>MNRQELITEALKARDMAYAPYSKFQVGAALLTKDGKVYRGCNIENAAYSMCNCAERTALFKAVSEGDTEFQMLAVA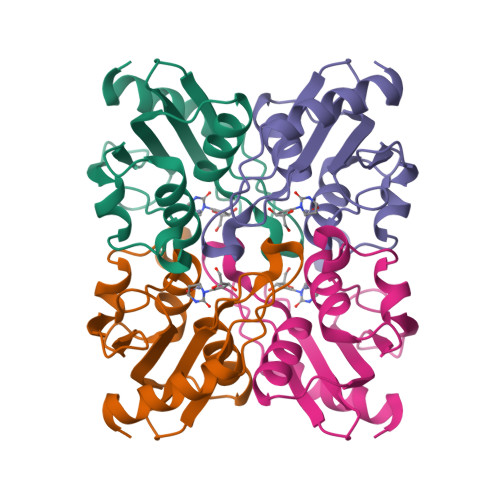ADTPGPVSPCGACRQVISELCTKDVIVVLTNLQGQIKEMTVEELLPGAFSSEDLHDERKL[2x]Acinetobacter sp. Ver3 is a polyextremophilic strain characterized by a high tolerance to radiation and pro-oxidants. The Ver3 genome comprises the sodB and sodC genes encoding an iron (AV3SodB) and a copper/zinc superoxide dismutase (AV3SodC), respectively; however, the specific role(s) of these genes has remained elusive. SODs are widely distributed diverse metalloenzymes that are classified according to the metal cofactor present in the active site. Manganese SODs (MnSODs or SodA enzymes) and iron SODs (FeSODs or SodB enzymes) are found in the bacterial cytosol and have very similar active sites, suggesting that these enzymes are closely related and evolved from a common ancestor, a relation that is supported by the identification of SOD variants termed cambialistic that use either iron or manganese (cambialistic Fe/MnSODs) depending on metal availability.

In order to explore the structural properties of AV3SodB, we solved the crystal structure of the enzyme to 1.34 Å resolution. AV3SodB crystallized in space group C2221, with one protein molecule per asymmetric unit. The final atomic model comprises AV3SodB residues 1–208. The Root-mean-square deviation (RMSD) between the AV3SodB monomer and the chain A in the E. coli FeSOD structure is 0.9 Å for 191 aligned residues. The active site of AV3SodB, located close to the dimer interface, is composed of conserved residues among FeSODs. mFo-DFc electron density maps clearly revealed the presence of a metal ion bound at the active site, which, based on our bioinformatic analysis, was modelled as an iron ion. The metal ion is coordinated in a distorted trigonal bipyramidal geometry with the side chain of His28 and a solvent molecule as axial ligands and the side chains of His80, Asp164 and His168 as equatorial ligands. The OH-/H2O ligand hydrogen bonds Asp164 and the active site Gln76. This OH-/H2O, believed to be OH- in oxidized FeSODs and H2O in the reduced enzymes, is connected to bulk water via a conserved hydrogen bonding network that begins with Gln76 and continues with residues Tyr36 and His32. Additional conserved hydrogen bonds link the active site to the interface between AV3SodB monomers, including a hydrogen bond between His32 of one monomer and Tyr171 of the other, and a hydrogen bond between His168 of one monomer and Glu167 of the other. Interestingly, AV3SodB crystallized in the presence of flavin mononucleotide (FMN), added as an additive in homemade crystallization conditions.

> MTTITLPALPYGYEDLAPHISKETLEYHHDKHHNTYVVNLNNLIAGTDLEGKTLEEIIKASVGDASKAGIFNNAAQVWNHTFYWNCMAKNGGGKATGALAAKIDEAFGSYEKFAEEFAAAATTQFGSGWAWLVADEVNGKLSIMKTSNADTPLAHGKVAVLTIDVWEHAYYIDFRNARPKYISTFLESLVNWDYANAKYAGQEAGVEK> MKLDIKKTFSNRSDRVKGIDFHPTEPWVLTTLYSGRVELWNYETQVEVRSIQVTETPVRAGKFIARKNWIIVGSDDFRIRVFNYNTGEKVVDFEAHPDYIRSIAVHPTKPYVLSGSDDLTVKLWNWENNWALEQTFEGHEHFVMCVAFNPKDPSTFASGCLDRTVKVWSLGQSTPNFTLTTGQERGVNYVDYYPLPDKPYMITASDDLTIKIWDYQTKSCVATLEGHMSNVSFAVFHPTLPIIISGSEDGTLKIWNSSTYKVEKTLNVGLERSWCIATHPTGRKNYIA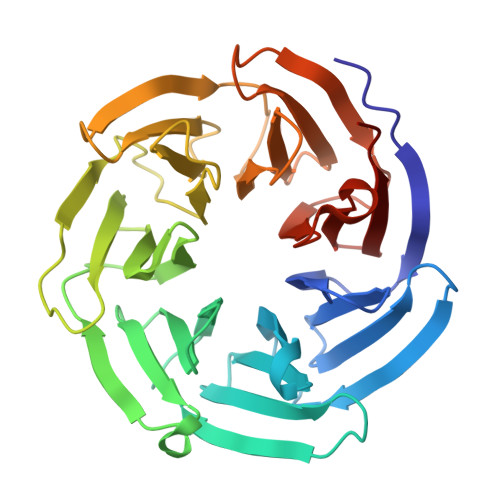SGFDNGFTVLSLGNDE>[2x]HHHHHHGSSQLLPAPLTNDPTAIGPVLPFEELHPRRYPENTATFLTRLRSLPSNHLPQPTLNCLLSAVSDQTKVSEEHLWESLQTILPDSQLSNEETNTLGLSTEHLTALAHLYNFQATVYSDRGPILFGPSDTIKRIDITHTTGPPSHFSPGK

We also reported that the TYMV papain-like cysteine PRO domain involved in the proteolytic processing of the viral replication precursor protein, also displays a DUB activity that was able to rescue the viral polymerase from degradation. The structure of the recombinant TYMV PRO/DUB domain we solved previously (residues 728–879 of the TYMV replication precursor protein) highlighted its homology with members of the ovarian tumor domain-containing (OTU) superfamily of DUBs. In addition, the TYMV PRO/DUB structure displayed a surprisingly exposed and minimal catalytic site, with a Cys783-His869 catalytic dyad instead of the conserved OTU DUB Cys-His-Asp/Asn catalytic triad. The structures reported herein reveal that the loop harboring the 865-GPP-867 motif is a highly mobile flap on the otherwise rigid PRO/DUB framework a result that is confirmed by molecular dynamics simulations.

In order to get an atomic view of a conformation of PRO/DUB not constrained by the crystal-induced PRO:PRO interaction, we generated a recombinant mutant harbouring deletion of the five C-terminal residues (hereafter ΔC5), corresponding to residues 728–874 of the TYMV 206K polyprotein. The ΔC5 crystal contains two molecules per asymmetric unit, hereafter referred to as molecules 'A' and 'B'. Clear electron density is present for residues 730–874 of molecule 'A', and 732–874 of molecule 'B'. Both molecules have their C-termini far from the catalytic sites of other molecules in the crystal packing. We thus have two independent views of PRO/DUB not engaged as a substrate in a PRO:PRO complex. Superimposition of molecules 'A' and 'B' of the ΔC5 mutant with the WT (engaged) PRO/DUB shows that PRO/DUB retains the same conformation in all three environments, with the exception of loop 864–868. In molecule 'B', Pro866 at the tip of the loop moves by 9 Å to a position overhanging the catalytic cleft. In fact, in molecule 'B', the mobility of this loop leads to the closure of a hydrophobic zipper between Pro866 and Pro867 on one side, and Leu820 and Leu781 across the catalytic cleft on the other side. His869 and Cys783 also come significantly closer together. However, it is clear that, in this closed conformation, His869 is now close enough to abstract a proton from Cys783. In summary, the crystal structure of ΔC5 indicates that, while TYMV PRO/DUB is a rigid molecule, it harbours a very mobile loop, 864-TGPPS-868, that can shift the GPP flap at its tip with its atypical double cis-proline, from an "open" state where it can be recognized by another PRO molecule, to two other states: a "closed" one where it forms half of a hydrophobic zipper, and an "intermediate" one, halfway in between.[[(2R,3S,4R,5R)-5-(6-aminopurin-9-yl)-3,4-dihydroxy-oxolan-2-yl]methoxy-hydroxy-phosphoryl] (2S)-2-azanyl-4-methylsulfanyl-butanoate | C15 H23 N6 O8 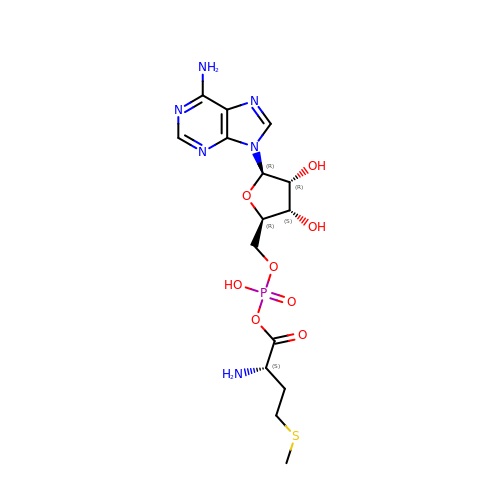P S | RZQLXQQLNKBFRX-TWBCTODHSA-N> GAMKITTWNVNSLNVRLPQV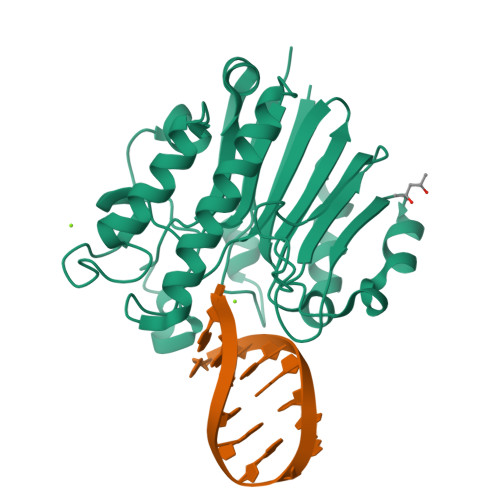QNLLADNPPDILVLQELKLDQDKFPAAALQMMGWHCVWSGQKTYNGVAIVSRSVPQDVHFGLPALPDDPQRRVIAATVSGVRVINVYCVNGEALDSPKFKYKEQWFAALTEFVRDEMTRHGKLVLLGNFNIAPADADCYDPEKWHEKIHCSSVERQWFQNLLDLGLTDSLRQVHPEGAFYTWFDYRGAMFQRKLGLRIDHILVSPAMAAALKDVRVDLETRALERPSDHAPVTAEFDW> LPVTVEKP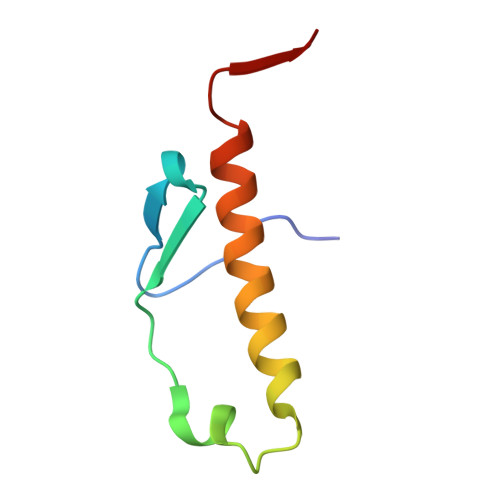IPVVYDLGNLAAFDSNVLDKNDLDSSNARREEKIKSLTRDNVQLLINQLLSLPMKTT>MGSTKPRFTTGLVYDTLMLKHQCTCGSSSSHPEHAGRIQSIWSRLQETGLRGKCECIRGRKATLEELQTVHSEAHTLLYGTNPANRQKLDSKKLLGSLASVFVRLPCGGVGVDSDTIWNEVHSAGAARLAVGCVVELVFKVATGELKNGFAVVRPPGHHAEESTPMGFCYFNSVAVAAKLLQQRLSVSKILIVDWDVHHGNGTQQAFYSDPSVLYMSLHRYDDGNFFPGSGAPDEVGTGPGVGFNVNMAFTGGLDPPMGDAEYLAAFRTVVMPIASEFAPDVVLVSSGFDAVEGHPTPLG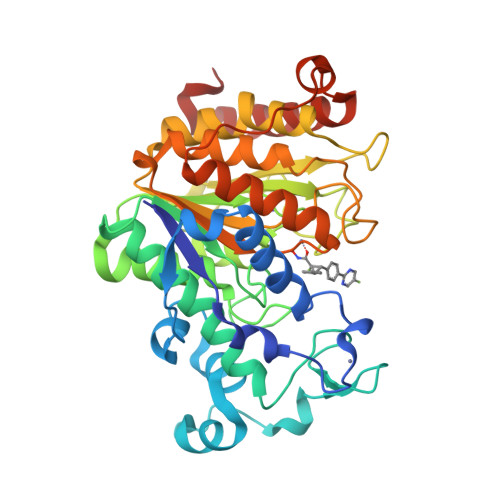GYNLSARCFGYLTKQLMGLAGGRIVLALEGGHDLTAICDASEACVSALLGNELDPLPEKVLQQRPNANAVRSMEKVMEIHSKYWRCLQRHHHHHH[2x]>[2x]MENSLFNQEVQIPLTESYCGPCPKNWICYKNNCYQFFDESKNWYESQASCMSQNASLLKVYSKEDQDLLKLVKSYHWMGLVHIPTNGSWQWEDGSILSPNLLTIIEMQKGDCALYASSFKGYIENCSTPNTYICMQRTV;> MEPHSLRYDFTVLSWDGSVQSGFLTEVHLDGQPFIRCDRQKCRAKPQGQWAEDVLGNKTWDRETRDLTGNGKDLRMTLAHIKD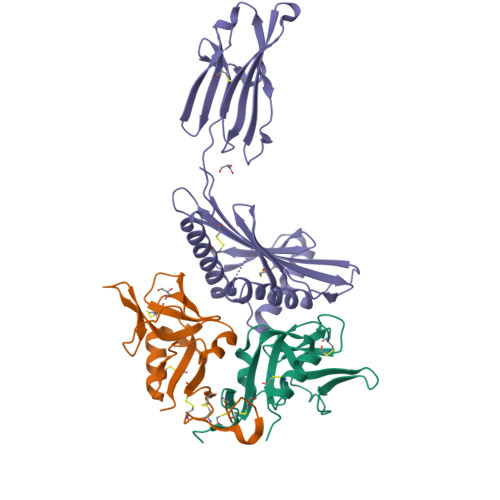QKEGLHSLQEIRVCEIHEDNSTRSSHHFYYDGELFLSWNLETKEFTMPQSSRAQTLAMNVRNFWKEDAMKTKTHFHAMRADCLQELRRYLKSGVILRRTVPPMVNVTRSEASEGNITVTCRASGFYPWNITLSWRQDGVSLSHDTQQWGDVLPDGNGTYQTWVATRICQGEEQRFTCYMEHSGNHSTHPVPS>[2x]GPLGSSGGDPARPGLSQQQRASQRKAQVRGLPRAKKLEKLGVFSACKANET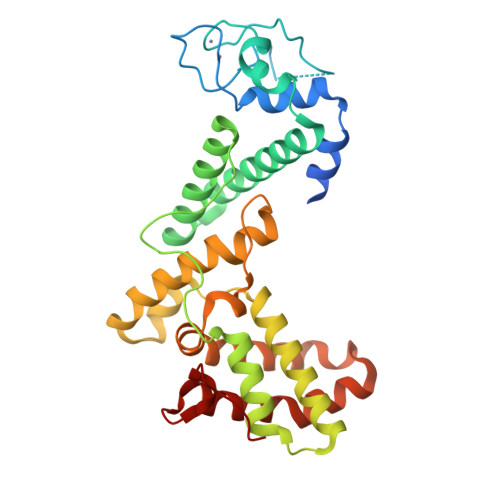CKCNGWKNPKPPTAPRMDLQQPAANLSELCRSCEHPLADHVSHLENVSEDEINRLLGMVVDVENLFMSVHKEEDTDTKQVYFYLFKLLRKCILQMTRPVVEGSLGSPPFEKPNIEQGVLNFVQYKFSHLAPRERQTMFELSKMFLLCLNYWKLETPAQFRQRSQSEDVATYKVNYTRWLCYCHVPQSCDSLPRYETTHVFGRSLLRSIFTVTRRQLLEKFRVEKDKLVPEKRTLILTHFPKFLSMLEEEIYGANSPIWESGFTMPP>[5x]HHHHHHMEIPSKQIDYRDVFIEFLTTFKGNNNQNKYIERINELVAYRKKSLIIEFSDVLSFNENLAYEIINNTKIILPILEGALYDHILQLDPTYQRDIEKVHVRIVGIPRVIELRKIRSTDIGKLITIDGILVKVTPVKERIYKATYKHIHPDCMQEFEWPEDEEMPEVLEMPTICPKCGKPGQFRLIPEKTKLIDWQKAVIQERPEEVPSGQLPRQLEIILEDDLV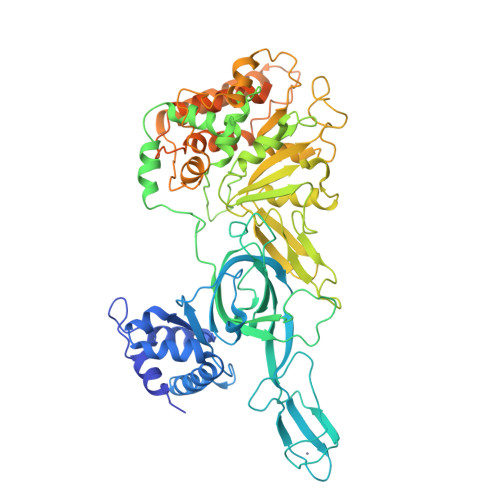DSARPGDRVKVTGILDIKQDSPVKRGSRAVFDIYMKVSSIEVSQKVLDEVIISEEDEKKIKDLAKDPWIRDRIISSIAPSIYGHWELKEALALALFGGVPKVLEDTRIRGDIHILIIGDPGTAKSQMLQFISRVAPRAVYTTGKGSTAAGLTAAVVREKGTGEYYLEAGALVLADGGIAVIDEIDKMRDEDRVAIHEAMEQQTVSIAKAGIVAKLNARAAVIAAGNPKFGRYISERPVSDNINLPPTILSRFDLIFILKDQPGEQDRELANYILDVHSGKSTKNIIDIDTLRKYIAYARKYVTPKITSEAKNLITDFFVEMRKKSSETPDSPILITPRQLEALIRISEAYAKMALKAEVTREDAERAINIMRLFLESVGVDMESGKIDIDTIMTGKPKSAREKMMKIIEIIDSLAVSSECAKVKDILKEAQQVGIEKSNIEKLLTDMRKSGIIYEAKPECYKKV> NESVRYDA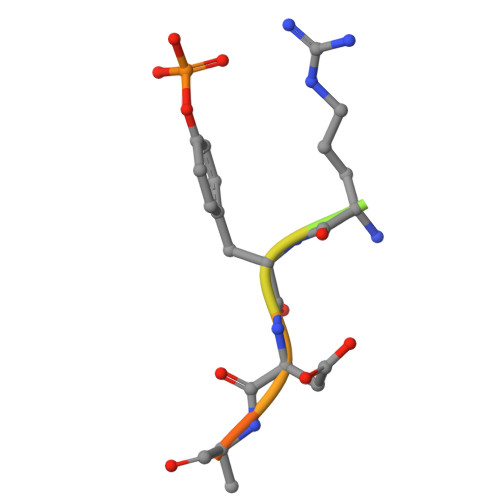TFP>[2x]NLGLDCDEHSSESRCCRYPLTVDFEAFGWDWIIAPKRYKANYCSGQCEYMFMQKYPHTHLVQQANPRGSAGPCCTPTKMSPINMLYFNDKQQIIYGKIPGMVVDRCGCS;>GNCWLRQAKNGRCQVLYKTELSKEECCSTGRLSTSWTEEDVNDNTLFKWMIFNGGAPNCIPCKETCENVDCGPGKKCRMNKKNKPRCVCAPDCSNITWKGPVCGLDGKTYRNECALLKARC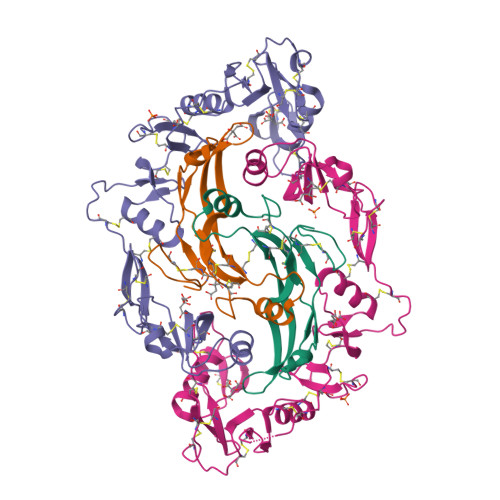KEQPELEVQYQGRCKKTCRDVFCPGSSTCVVDQTNNAYCVTCNRICPEPASSEQYLCGNDGVTYSSACHLRKATCLLGRSIGLAYEGKCIKAKSCEDIQCTGGKKCLWDFKVGRGRCSLCDELCPDSKSDEPVCASDNATYASECAMKEAACSSGVLLEVKHSGSCN[2x]> GP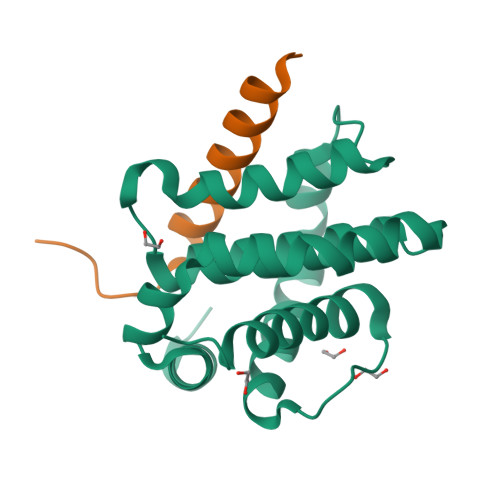LGSMDEDVLPGEVLAIEGIFMACGLNEPEYLYHPLLSPIKLYITGLMRDKESLFEAMLANVRFHSTTGINQLGLSMLQVSGDGNMNWGRALAILTFGSFVAQKLSNEPHLRDFALAVLPAYAYEAIGPQWFRARGGWRGLKAYCTQVLT;> SESQEDIIRNIARHLAQVGDSMDRSIPPGLVNGL> AEIKNLIDRGTYRKLPLFEGELPEGSYAQIVEVKPKQTVKKHYHERQYELFYIISGEARLGIGDTEYQAKPGDIFLVKPKTVHWVVNEKDEPFRLFVVKLNYHGDDSVWLEGS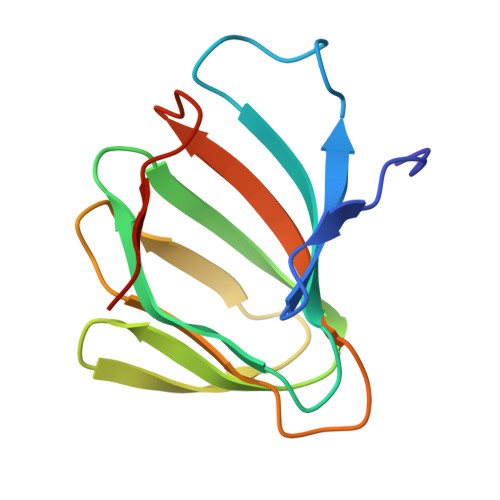F>[2x]MPNSEPASLLELFNSIATQGELVRSLKAGNASKDEIDSAVKMLVSLKMSYKAAAGEDYKADCPPGNPAPTSNHGPDATEAEEDFVDPWTVQTSSAKGIDYDKLIVRFGSSKIDKELINRIERATGQRPHRFLRRGIFFSHRDMNQVLDAYENKKPFYLYTGRGPSSEAM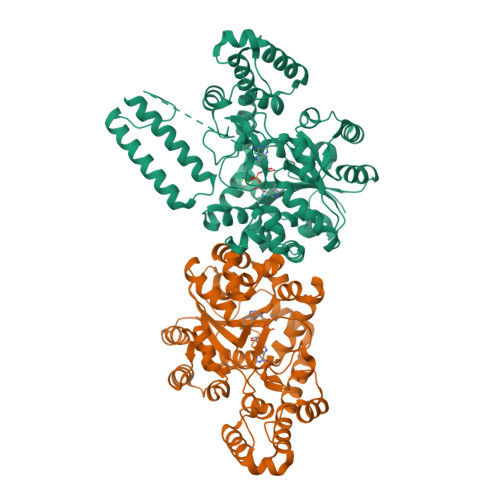HVGHLIPFIFTKWLQDVFNVPLVIQMTDDEKYLWKDLTLDQAYSYAVENAKDIIACGFDINKTFIFSDLDYMGMSSGFYKNVVKIQKHVTFNQVKGIFGFTDSDCIGKISFPAIQAAPSFSNSFPQIFRDRTDIQCLIPCAIDQDPYFRMTRDVAPRIGYPKPALLHSTFFPALQGAQTKMSASDPNSSIFLTDTAKQIKTKVNKHAFSGGRDTIEEHRQFGGNCDVDVSFMYLTFFLEDDDKLEQIRKDYTSGAMLTGELKKALIEVLQPLIAEHQARRKEVTDEIVKEFMTPRKLSFDFQKLAAALEHHHHHH>MEGGKLQSTFVFEEIGRRLKDIGPEVVKKVNAVFEWHITKGGNIGAKWTIDLKSGSGKVYQGPAKGAADTTIILSDEDFMEVVLGKLDPQKAFFSGRLKARGNIMLSQKLXMILKDYAKLGSENLYFQ[2x]

The Kamer and Jarvis groups have extensively studied the human steroid carrier protein (SCP-2L),23 a single-domain 13.5 kDa protein containing a hydrophobic tunnel, as a scaffold for ArM design. The steroid carrier protein type 2 like (SCP-2L) domain of the human multifunctional enzyme 2 (MFE-2) has previously been used as a protein scaffold for both regioselective and enantioselective reactions using covalent modification through the introduction of unique cysteine residues. Here two methods for site-selective incorporation of bipyridine into the SCP-2L scaffold were compared, and the copper-catalysed 1,4-addition of indole to enones was used to analyse ArM activity. Crystals of SCP_Q111CBpy and SCP_Q111BpyAla were soaked in solutions of Cu(ii) ions and their structures determined by X-ray crystallography.

The structure of Cu(ii)-bound SCP_Q111BpyAla was determined to 2.51 Å resolution and revealed a different orientation of the bipyridine moiety compared to that seen in the Cu(ii)-bound SCP_Q111CBpy structure. Despite the lower resolution, the electron density for the BpyAla bipyridine rings, α-helix 5 and the additional C-terminal amino acids (120–128) was very clear, indicative of a more rigid conformation for these parts of the protein. The co-planar BpyAla bipyridine rings are wedged into a shallow pocket formed by the turn between G85 and P89 at the edge of the apolar tunnel. This conformation is stabilised by van der Waals interactions between C1 of BpyAla and both G85 Hα (3.35 Å) and D88 Hα (3.36 Å), C2 of BpyAla and Hδ of P89 (2.87 Å: 3.36 Å to the Cδ) and C3 of BpyAla and Hγ of P89 (2.74 Å: 3.26 Å to the Cγ). In addition, the side-chains of D88 and K115 (one turn down on α-helix 5) lie on either face of the bipyridine and may stabilise the BpyAla conformation by aromatic–π electrostatic interactions. The B-factors for the Bpy moiety and the Cu(ii) ion (43 Å2 and 57.91 Å2, respectively) were lower in this structure compared to the bipyridine rings in the Cu(ii)-bound Q111CBipy structure, indicating that the catalytic environment is more rigid. Among the novel ArMs, SCP_Q111BpyAla displayed the greatest enantioselectivity with an e.r. of 20 : 80 (±1), favouring the S enantiomer, and a yield of 42% (entry 9). Overall, the substrates' activation in FC alkylation mechanism with SCP_Q111BpyAla favours the formation of proS product over proR while with SCP_Q111CBpy favours proR product formation over proS. The crystal structure obtained of SCP-Q111BpyAla_Cu is a rare example of a protein structure containing an unnatural amino acid.4-({4-[(4-{4-[(E)-2-cyanoethenyl]-2,6-dimethylphenoxy}thieno[3,2-d]pyrimidin-2-yl)amino]piperidin-1-yl}methyl)benzene-1-sulfonamide | C29 H30 N6 O3 S2 | 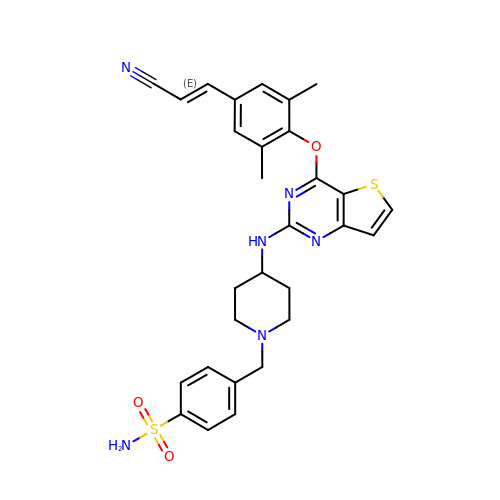GVCHBMCBPBRORW-ONEGZZNKSA-N>[2x]KFGWIKGVLVRCMLNIWGVMLFIRMTWIVGQ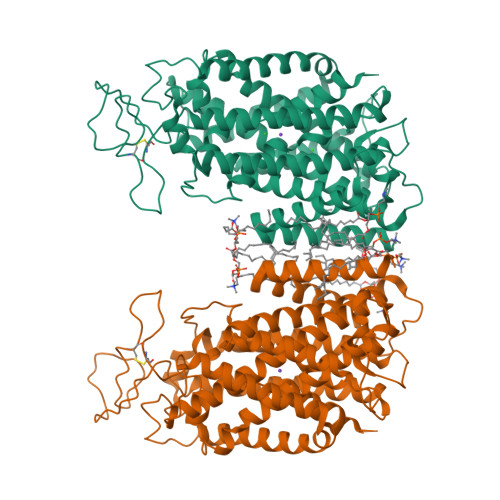AGIAYSCIIVIMATVVTTITGCSTSAIATNGFVRGGGAYYLISRSLGPEFGGSIGLIFAFANAVAVAMYVVGFAETVVELLMDSGLLMIDQTNDIRVIGTITVILLLGISVAGMEWEAKAQIFLLVILITAIFNYFIGSFIAVDSKKKFGFFSYDAGILAENFGPDFRGQTFFSVFSIFFPAATGILAGANISGDLADPQMAIPKGTLLAILITGLVYVGVAISAGACIVRDATGIESNFTLISNCTDAACKYGYDFSSCRPTVEGEVSSCKFGLHNDFQVMSVVSGFSPLISAGIFSATLSSALASLVSAPKVFQALCKDNIYPGIAIFGKGYGKNNEPLRGYFLTFGIALAFILIAELNVIAPIISNFFLASYALINFSVFHASLANSPGWRPSFKYYNMWASLAGAILCCVVMFIINWWAALLTNVIVLSLYIYVSYK Each of these enzymes catalyzes as their main activity the cyclization of N-γ-acetyl-L-2,4-diaminobutyric acid (N-γ-ADABA), the reaction product of the 2,4-diaminobutyrate acetyltransferase (EctA), to ectoine with the concomitant release of a water molecule. We demonstrate here for the first time that the ectoine synthase is a metal-dependent enzyme, with iron as the most likely physiologically relevant co-factor. The EctC protein forms a dimer in solution and our structural analysis identifies it as a member of the cupin superfamily. The two crystal structures that we report here for the (Sa)EctC protein (with resolutions of 1.2 Å and 2.0 Å, respectively), and data derived from extensive site-directed mutagenesis experiments targeting evolutionarily highly conserved residues within the extended EctC protein family, provide a first view into the architecture of the catalytic core of the ectoine synthase.

Crystal form A diffracted to 1.2 Å and had a unit cell of a = 72.71 b = 72.71 c = 52.33 Å and α = 90 β = 90 γ = 120° displaying a P3221 symmetry. Finally, a monomer of this structure was used as a template for molecular replacement to phase the high-resolution (1.2 Å) dataset of crystal form A, which was subsequently refined to a final Rcryst of 12.4% and an Rfree of 14.9%. First, the 1.2 Å structure reveals the spatial configuration of the (Sa)EctC protein ranging from amino acid Met-1 to Glu-115; hence, it lacks 22 amino acids at the carboxy-terminus of the authentic (Sa)EctC protein. This structure adopts an open conformation with respect to the typical fold of cupin barrels and is therefore termed in the following the “open” (Sa)EctC structure. In this structure no metal co-factor was identified. In the “open” (Sa)EctC structure, one monomer is present in the asymmetric unit. Indeed, a similar dimer configuration to the one described for the “semi-closed” (Sa)EctC structure is observed with the same monomer-monomer interactions mediated by the two β-sheets. In the “open” (Sa)EctC structure, both proline residues are visible in the electron density; however, almost directly after Pro-110, the electron density is drastically diminished caused by the flexibility of the carboxy-terminus. In the “open” structure of the (Sa)EctC protein, this interaction does not occur since Glu-115 is rotated outwards. However, this electron density fits perfectly to a water molecule and not to an iron, and the water molecule was clearly visible after the refinement at this high resolution (1.2 Å) of the “open” (Sa)EctC structure.

> MIVRNLGDIRKTDRNVRSDGWASARMLLKDDGMGFSFHVTTLFAGSELRMHYQNHLEAVLVLKGTGTIEDLATGEVHALRPGVMYALDDHDRHIVRPETDILTACVFNPPVTGREVHDESGAYPADPELAREPVAADNWSHPQFEK> MPRRSARKAQSAIASPADTNVVPAKDAPTTNSPPSTTSPNQAAADANQQQAGIVSSQSGPNAVGDSAPSSSVNNDGDIITRPTSDSIAAVANATKPAAVVSDPQSMKVTPIVNPSSYVCNVCNARFSTMSALSEHLRSDHRDDASTLLATPMINNAIRSFLTAWDDIRILSPDVSSKSLSAYLDSAVANGPELIIEDTGLCTSFMLLDNIPSAHLTKELIGFTWFMQMYQMTPPLPEGAVNRIVCMTNWASLGDEGRGLEVRLPPPTDSSVHAYKTVLSRGYIDNAQFNPLALRSNVLLMLLQFTLSNLKINKSSTFTSDVTTITSGRMIRAFEGRPELLALAYPGRAVLPTQTKNAQFLSTAIADRIGRLDRANLIGGEVSAMVECMELCDALTLHIRETYIMLLRSMHQDPTQIVQIVNECANNLLNSTIPISLRPTILCPWFASSEDLRLQQVMHLVNISSNTAAALPLVEALSTLLRSVTPLVLDPTVLTNAITTISESTTQTISPISEILRLLQPMGNDYAAFWKCIASWAYNGLVTTVLSEDAFPDSSQSITHLPSMWKCLFLTLAGPMTSDPHSPVKVFMALANLLAQPEPIAIGVPGMHQTTPASQFSHPGVWPPGFLNPQLINPQQAPLLRAFAEHIRANWPQPSEFGYGSTLQGSANLFIPSNRMVYPWPNQPLPRLTVAPTYDSAMSNWISTTIAFFIRVVNSVNMTATVNDLTRRTMTGVMTAMRQVKTMTPFYIQHMCPTELSVLASVTVTPPFQVPFTRLVQNDVITNVLVARVDPAQRGDAAVDIRATHATFAAALPVDPAAIVVAMLCGQTETNLIPSHHYGKAFAPLFASNAMFTRNQRAVITREAFVCARSAVAQCQDAGFLVPRPLDALRQFDVTSAAAAEIMHAVNDAFKTAFDLDGALLDGLALYGDPRIADLSAAYLQYGGNVVREHVPPGPSHIHRALQQVESTFMAEMNLFNVARGNLYLVQTATNGNWSPMAPVAAPPFVRGGPNVRVVGRFGTIVPRPNGLEPQLIDDGNVPRDIAGDWVYPSDVLQVSVAVFRDYVWPMVKAGRTRVLVELGHYVYTLHYYDPQISLDEAPILEEWLSKINPAGIPPVPFCIPIPQVYPCITARRVHYAFTSENNNDSLFSTNAASIDTAFGENAAVSPLRWPGLVDPNYRVGTNDLPNRITLYNSLYRYNFTYPTLDGIMYV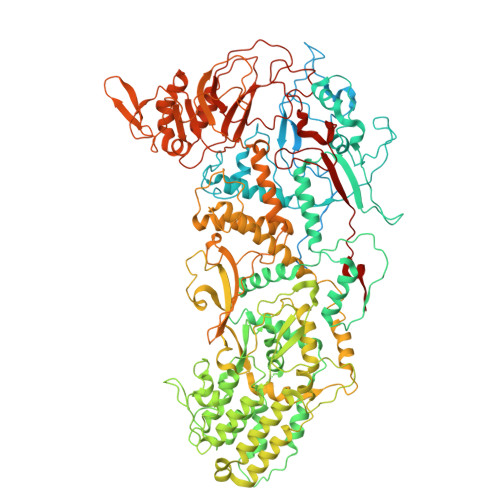RSAT>[2x]GSHNMAEMVETVCGPVPVEQLGKTLIHEHFLFGYPGFQGDVTRGTFREDESLRVAVEAAEKMKRHGIQTVVDPTPNDCGRNPAFLRRVAEETGLNIICATGYYYEGEGAPPYFQFRRLLGTAEDDIYDMFMAELTEGIADTGIKAGVIKLASSKGRITEYEKMFFRAAARAQKETGAVIITHTQEGTMGPEQAAYLLEHGADPKKIVIGHMCGNTDPDYHRKTLAYGVYIAFDRFGIQGMVGA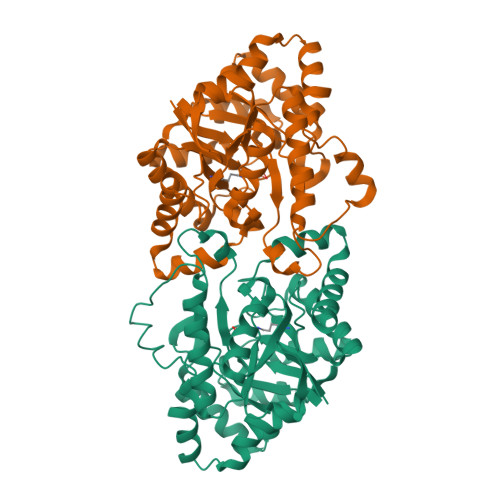PTDEERVRTLLALLRDGYEKQIMLSHDTVNVWLGRPFTLPEPFAEMMKNWHVEHLFVNIIPALKNEGIRDEVLEQMFIGNPAALFSA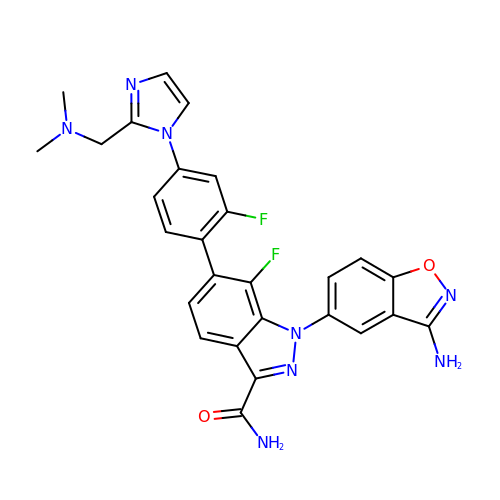1-(3-amino-1,2-benzisoxazol-5-yl)-6-(4-{2-[(dimethylamino)methyl]-1H-imidazol-1-yl}-2-fluorophenyl)-7-fluoro-1H-indazole-3-carboxamide | C27 H22 F2 N8 O2 | MGUDDBRJHXFTEY-UHFFFAOYSA-N> LVH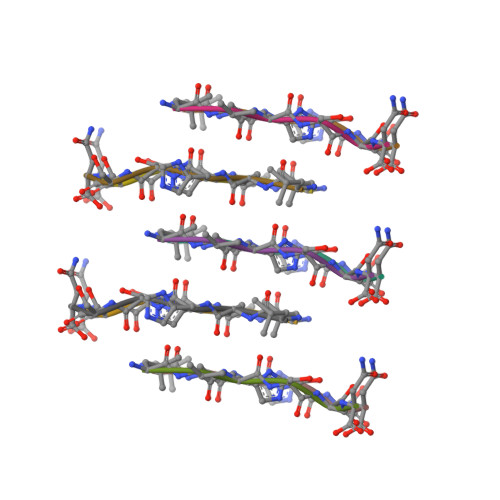SSN>MKNLRYKLLLFVFIGFWGLLALNLFILSVKNQEYYEKLAERNMTKKEFLVPTRGNITDRNDEFLATNELVFGVFLPSGLKQKDLLEKIEIIQKFFPNFSKETLLNNYQKENSLYNHNLIKVVGFIPYATMQPLYAKLIQTQGIFALPLDKRYYPNNALASHVLGYVGVASLQDLKDDEENQYSQIVGKTGIEKEYNKLLQGKVGYKIMRVNALNQELATLEVVLPSTNNHLQLSLDKRLQKEADKLFENKRGAILVMDAENGELLVAGSYPEYNLNDFVGGISQDKWQKLQDDIYNPLLNRFANALYPPGSVVKMGVGLSFLENLHITENTTIPTPPFIEVGKHKFRDWKKTGHGNSNLYKAIRESVDVYFYKFGLEISIEKLSKTLREVGFGEKTGVDLPNEFVGIVPDNLWKLKRFNQDWRVGDTLITAIGQGSFLATPLQVLAYTGLIATGKLATPHFAINNKQPLKDPLNSFQKKKLQALRVGMYEVCNHKDGTAYHSTRGSKITLACKTGTAQVVEIAQNIVNRMKEKDMEYFHRSHAWITAFLPYEKPKYAITILVEHGEGGSKLGGLLVKMSNKLYELGYLHHHHHH[2x];>[4x]MRFYFKFLWLLGIFLIFYFLDFKGSSSYISDRIKNALMNAKNSLLDNVQAYFFQAQNIKEFQKERLILEALKLENADLKERLNSIYPLENPKMTYTPTFMTSFISLEDTHSVSLNPIVNLEENKIYGLVSHNQAIGIAVLEKGRLNGFLNAHKRCAYSVMIGQNQVLGFIGTNFKQELVVDFIVPSAEINIGDQVLTSGLDGIFGAGVFVGEVSSIEDHYTYKSAVLKNAFLSGAKLLRHVFLSDVKN

Penicillin-binding proteins (PBPs) catalyze the two last reactions in PG biosynthesis (GlcNAc-MurNAc polymerization and stem peptide cross-linking, or transpeptidation). Class A enzymes can catalyze both reactions, while class B PBPs act uniquely as transpeptidases. Within the elongasome of a variety of bacteria including E. coli, Caulobacter crescentus, Bacillus subtilis, and Helicobacter pylori, PBPs have been shown to interact with, and be recruited by, the essential protein MreC, a bitopic membrane protein that is essential for cell shape. PBP2 (residues L38–L588, thus lacking the TM helix) is a 588-residue molecule that presents the characteristic fold of class B PBPs, with an elongated N-terminal region followed by a transpeptidase domain that carries the stem peptide cross-linking site.

PBP2:MreC complex crystals yielded diffraction data to 2.7 Å and harbored two 1:2 PBP2:MreC complexes in the asymmetric unit. Diffraction data were phased by using our structure of PBP2 from H. pylori as a model in a molecular replacement experiment. Two “butterflies” are present in the asymmetric unit of the complex, but only one interacts directly with PBP2, the other one interacting uniquely with its partner MreC. Thus, MreC employs two distinct surfaces for partner molecule recognition, a fact that relates directly to its biological role of scaffold protein. MreC interacts with PBP2 by inserting its C-terminal β-domain between the head and anchor regions of the PBP, forcing the anchor region to “sway” by ~15 Å away from the head. The swaying movement is guaranteed by the flexibility of loops 50′–52′, 203′–204′, and 224′–227′ that act as a hinge, opening up the N-terminus into a “V” shape that accommodates MreC snugly. Direct interactions involve mostly the head region of PBP2, which recognizes MreC through a hydrophobic zipper generated by surface-exposed non-polar residues on both faces. These include Phe169, Phe182, and Tyr222 (MreC); Leu69′, Phe71′, Tyr127′, and Tyr134′ (PBP2); Phe169 (MreC); and Tyr134′ (PBP2), forming a π–π stacking pair. The fact that hydrophobic interactions (more feeble than polar interactions) are involved in PBP2:MreC recognition indicates that these complexes can form and be disrupted as needed during the cell wall elongation process.> ASMQKLINSVQNYAWGSKTALTELYGIANPQQQPMAELWMGAHPKSSSRITTANGETVSLRDAIEKNKTAMLGEAVANRFGELPFLFKVLCAAQPLSIQVHPNKRNSEIGFAKENAAGIPMDAAERNYKDPNHKPELVFALTPFLAMNAFREFSDIVSLLQPVAGAHSAIAHFLQVPNAERLSQLFASLLNMQGEEKSRALAVLKAALNSQQGEPWQTIRVISEYYPDDSGLFSPLLLNVVKLNPGEAMFLFAETPAA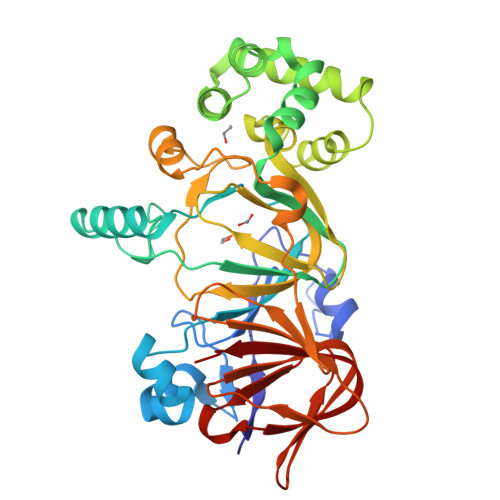YLQGVALEVMANSDNVLRAGLTPKYIDIPELVANVKFEPKPAGELLTAPVKSGAELDFPIPVDDFAFSLHDLALQETSIGQHSAAILFCVEGEAVLRKDEQRLVLKPGESAFIGADESPVNASGTGRLARVYNKL> MQDPDGIDINTKIFNSVAEVFQKAQGSYAGHRKHIAVLKKIQSKAVEQGYEDAFNFWFDKLVTKILPLKKNEIIGDRIVKLVAAFIASLERELILAKKQNYKLTNDEEGIFSRFVDQFIRHVLRGVESPDKNVRFRVLQLLAVIMDNIGEIDESLFNLLILSLNKRIYDREPTVRIQAVFCLTKFQDEEQTEHLTELSDNEENFEATRTLVASIQNDPSAEVRRAAMLNLINDNNTRPYILERARDVNIVNRRLVYSRILKSMGRKCFDDIEPHIFDQLIEWGLEDRELSVRNACKRLIAHDWLNALDGDLIELLEKLDVSRSSVCVKAIEALFQSRPDILSKIKFPESIWKDFTVEIAFLFRAIYLYCLDNNITEMLEENFPEASKLSEHLNH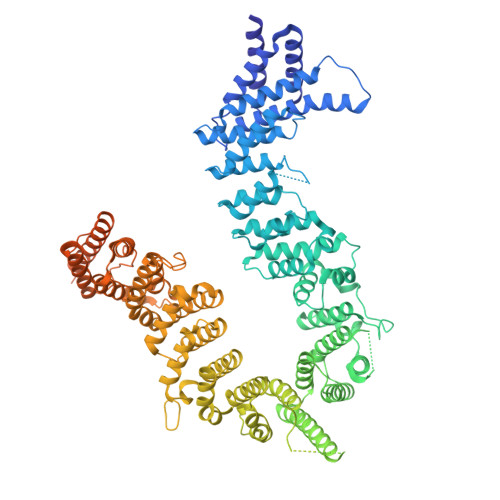YILLRYHHNDISNDSQSHFDYNTLEFIIEQLSIAAERYDYSDEVGRRSMLTVVRNMLALTTLSEPLIKIGIRVMKSLSINEKDFVTMAIEIINDIRDDDIEKQEQEEKIKSKKINRRNETSVDEEDENGTHNDEVNEDEEDDNISSFHSAVENLVQGNGNVSESDIINNLPPEKEASSATIVLCLTRSSYMLELVNTPLTENILIASLMDTLITPAVRNTAPNIRELGVKNLGLCCLLDVKLAIDNMYILGMCVSKGNASLKYIALQVIVDIFSVHGNTVVDGEGKVDSISLHKIFYKVLKNNGLPECQVIAAEGLCKLFLADVFTDDDLFETLVLSYFSPINSSNEALVQAFAFCIPVYCFSHPAHQQRMSRTAADILLRLCVLWDDLQSSVIPEVDREAMLKPNIIFQQLLFWTDPRNLVNQTGSTKKDTVQLTFLIDVLKIYAQIEKKEIKKMIITNINAIFLSSEQDYSTLKELLEYSDDIAENDNLDNVSKNALDKLRNNLNSLIEEINERSETQTKDENNTANDQYSSILGNSFNKSSNDTIEHAADITDGNNTELTKTTVNISAVDNTTEQSNSRKRTRSEAEQIDTSKNLENMSIQDTSTVAKNVSFVLPDEKSDAMSIDEEDKDSESFSEVC Most of the Mg2+ influx into mitochondria is mediated by the Mitochondrial RNA Splicing 2 (MRS2) channel, located in the inner mitochondrial membrane. MRS2 belongs to the CorA protein superfamily characterized by a highly conserved Glycine-Methionine-Asparagine (GMN) motif in the loop between transmembrane helix 1 and 2. MRS2 assembles into a homo-pentamer and displays an overall architecture similar to structures in the CorA family, with slight differences in the secondary structure arrangement. Along the pore, R332 and M336 have been identified as the main gating residues.

Four Mg2+ ions (termed Mg2+−1, 2, 3, 4) were identified along the pore and two (termed Mg2+−5, 6) were found in between neighboring soluble domains in the MRS2-Mg2+ structures. The upper most Mg2+ (Mg2+-1), closest to the mitochondrial intermembrane space is coordinated by the highly conserved GMN motif. Mg2+-1 interacts with a ring of backbone carbonyl oxygens of G360 and amine group of N362 with a distance of 3.8 Å and 4.3 Å, respectively, indicating that the Mg2+-1 is in hydrated form. Mg2+-2, Mg2+-3 and Mg2+-4 are coordinated by a ring of hydroxyl oxygens of T346, carbonyl oxygens of N339, and carboxylic oxygens of D329 with a distance of 5.2 Å, 4.3 Å and 3.5 Å, respectively. The radius plot estimated by the program HOLE37 shows the narrowest region of the pore is formed by a ring of M336 side chains, with a pore radius of 1.7 Å, followed by R332, and N362/G360, which is part of GMN motif. Two additional Mg2+ ions (Mg2+-5 and Mg2+-6) have been identified in the interface of neighboring subunits between their soluble N-terminal domains termed soluble sites 1 and 2. Mg2+-5 in site 1 interacts with side chains of T246, D247, E138, carboxyl oxygen of E243, and E312 from the neighboring subunit. Mg2+-6 in site 2 is sandwiched between two negatively charged glutamate clusters from two adjacent subunits. When overlaying the HsMRS2 structure to the archaeal MjCorA X-ray structure, in which 28 Mg2+ ions were modeled into the soluble domain in an asymmetric manner, the Mg2+ (atom spec: MgE406) between subunit E and A of MjCorA is close to soluble site 1 in MRS2; however, it is coordinated by E155, Y186, T90 and Q62, which is different to the groups of negatively charged residues (E138, E243, D247, E312) in MRS2. Interestingly, adjacent to soluble site 2 of HsMRS2, a salt bridge is observed between R116 from one subunit and E291 from the neighboring subunit, with a distance of 2.7–2.8 Å.

>[5x]MECLRSLPCLLPRAMRLPRRTLCALALDVTSVGPPVAACGRRANLIGRSRAAQLCGPDRLRVAGEVHRFRTSDVSQATLASVAPVFTVTKFDKQGNVTSFERKKTELYQELGLQARDLRFQHVMSITVRNNRIIMRMEYLKAVITPECLLILDYRNLNLEQWLFRELPSQLSGEGQLVTYPLPFEFRAIEALLQYWINTLQGKLSILQPLILETLDALVDPKHSSVDRSKLHILLQNGKSLSELETDIKIFKESILEILDEEELLEELCVSKWSDPQVFEKSSAGIDHAEEMELLLENYYRLADDLSNAARELRVLIDDSQSIIFINLDSHRNVMMRLNLQLTMGTFSLSLFGLMGVAFGMNLESSLEEDHRIFWLITGIMFMGSGLIWRRLLSFLGRQLEAPLPPMMASLPKKTLLADRSMELKNSLRLDGLGSGRSILTNRDYKDDDDK>[2x]MADIYIPTLEEIKRTLQLAKDYSENVYFIYRIALESGVRLSEILKVLKEPERDICGNDVCYYPLSWTRGYKGVFYVFHITPLKRVE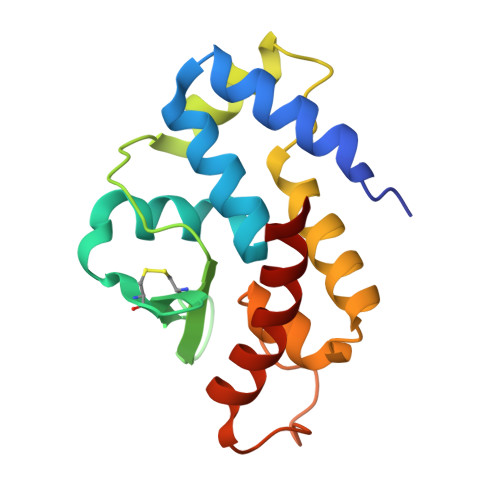VTKWAIADFERRHKDAIAIKYFRKFVASKMAELSVPLDIIDFIQGRKPTRVLTQHYVSLFGIAKEQYKKYAEWLKGV(2S)-2,3-dihydroxypropyl 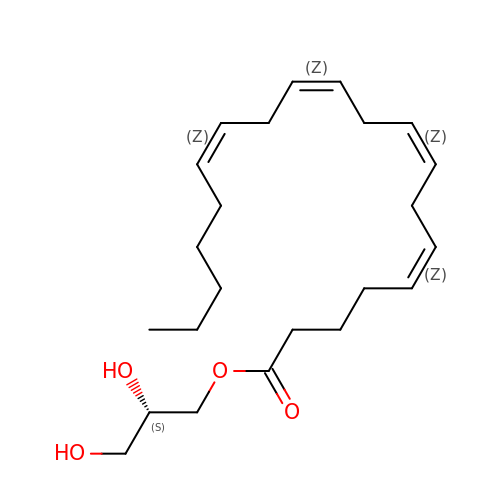(5Z,8Z,11Z,14Z)-icosa-5,8,11,14-tetraenoate | C23 H38 O4 | DCPCOKIYJYGMDN-HUDVFFLJSA-N> GAGAATTCCTGACGGAAATTA;>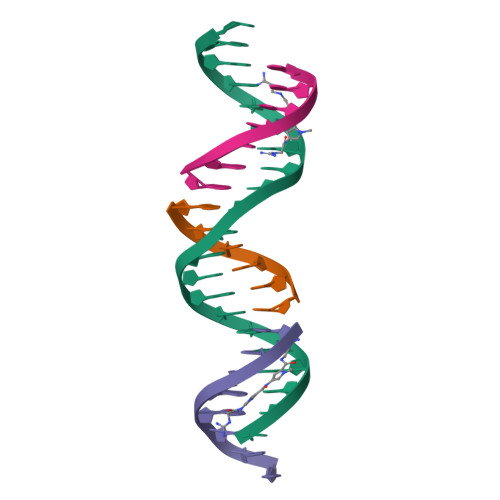 CCGTCA;> TCTAATTT;> GGAATTC> ELPDFFQGKHFFLYGEFPGDE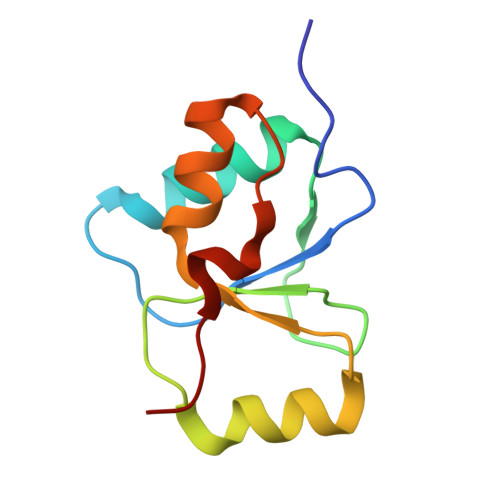RRKLIRYVTAFNGELEDYMSDRVQFVITAQEWDPSFEEALMDNPSLAFVRPRWIYSCNEKQKLLPHQLYGVVPQA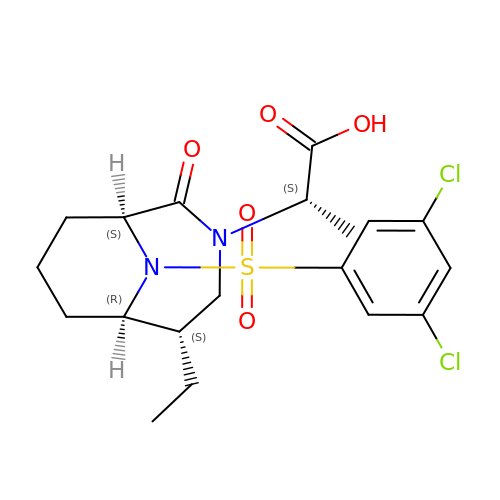(2~{S})-2-[(1~{S},5~{S},6~{R})-10-[3,5-bis(chloranyl)phenyl]sulfonyl-5-ethyl-2-oxidanylidene-3,10-diazabicyclo[4.3.1]decan-3-yl]propanoic acid | C19 H24 Cl2 N2 O5 S | NNQRIRRUEIVSQY-NQERCMRGSA-N> SACPSGATCGSYTVGGLGSRKQQVRNAGGSSLDLAVAMLETERMDTAYPYGDNKSGDAANFG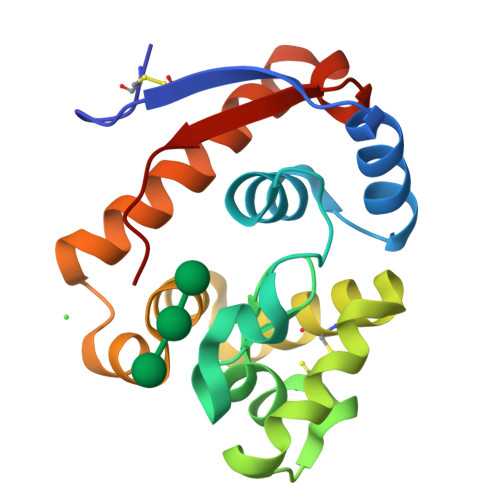IFKQNWLMLRSACAQFGGQGAGQYDNGAALNSSLGQDVSCLHQSQSHYGLDAWFAGHRNGASGLSSPNTADIAAYKAAVYWIKAQLDADSANLGNDTRFWVQVPAI> MTGIPPIPLLRLDPGIPVPVRAHEGDAGVDLCTTEDVIIEPGERVLVGTGIAVALPIGTVGLIHPRSGLAAKAGLSVVNTPGTVDAGYRGEIKVCLINHDPRAAIELRRGDRIAQLLVQKVELVDFVEVETLDETARGAGGYGSSGGHASLAAQSGGAGQATGKEAGGGGSLEVLFQGPGGGGSLEVDHHHHHH

Deoxyuridine 5′-triphosphate nucleotidohydrolase (dUTPase) is an enzyme encoded in nearly all prokaryotes, eukaryotes, and a majority of viruses. The enzyme catalyses the hydrolysis of dUTP to dUMP, eventually controlling the cellular dUTP:dTTP concentration to the level that could prevent incorporation of dUTP into DNA, which would overwhelm the DNA repair system, leading to multiple DNA strand breaks and eventually, cell death. N. seriolae dUTPase (NsdUTPase) plays a key role in the proliferation of Nocardia, and was regarded as a potent drug target. Among them, N. seriolae was identified as the main cause of fish nocardiosis, which lead to severe economic losses in the aquaculture industry.

We expressed and purified NsdUTPase in E. coli, and resolved its first crystal structure with a resolution of 2.12 Å. Purified NsdUTPase was crystallised in 25% (w/v) polyethylene glycol-3350 and 0.1 M Tris–HCl pH 8.5. Resolved NsdUTPase crystal structure showed a classical trimer assembling, and each dUTPase monomer is an asymmetry unit folding into a jelly-roll β-barrel structure, composed of a total of 11 β-strands grouped into four antiparallel β-sheets in addition to a single short α-helix between the fourth and fifth β-sheets. The structure alignment showed that although NsdUTPase exhibited similar folding pattern with dUTPases from M. tuberculosis (MtdUTPase) and M. abscessus (MadUTPase), there were still some differences between their conformations. Trimeric NsdUTPase contained three identical ligand binding sites located at clefts between adjacent monomers. And dUMP bound in the cleft of two monomers interacts with two monomers. Then, we verified the detailed interactions between dUMP and NsdUTPase, the uracil group of dUMP formed hydrogen bonds with the main chain of Ile92 and Lys93 as well as the side chain of Asn79. The phosphate group of dUMP formed hydrogen bond with the side chain of Ser67. In addition, dUMP showed hydrophobic interactions with a series of surrounding residues, including Ile63, Ile92, Lys93, and Tyr88. The active site of NsdUTPase was located in the surface, and consists of a series of hydrophobic interactions, which might be a promising binding pocket for ligand binding.> GSMENTDVFLGLHDFLERMRKPSAGDFVKSI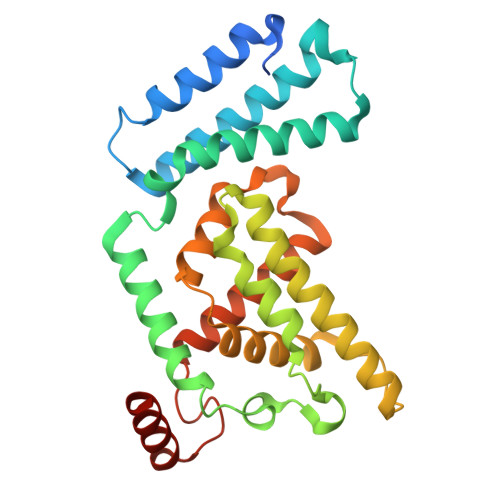KSFIVSFSNNAPDPEKDCAMVQEFFSKMEAAFRAHPLWSGCSEEELDSAGDGLEKYVMTKLFTRVFASNTEEVIADEKLFQKMSLVQQFISPENLDIQPTFQNESSWLLAQKELQKINMYKAPRDKLVCILNCCKVINNLLLNASIASNENAPGADEFLPVLIYVTIKANPPQLHSNLLYIQRYRRESKLVGEAAYFFTNILSAESFISNIDAKSISLDEAEFEKNMESARARISG>MGSHHHHHHTQPMPGKPAEDAENELDIRGLFRTLWAGKLWIIGMGLAFALIALAYTFFARQEWSSTAITDRPTVNMLGGYYSQQQFLRNLDVRSNMASADQPSVMDEAYKEFVMQLASWDTRREFWLQTDYYKQRMVGNSKADAALLDEMINNIQFIPGDFTRAVNDSVKLIAETAPDANNLLRQYVAFASQRAASHLNDELKGAWAARTIQMKAQVKRQEEVAKAIYDRRMNSIEQALKIAEQHNISRSATDVPAEELPDSEMFLLGRPMLQARLENLQAVGPAFDLDYDQNRAMLNTLNVGPTLDPRFQTYRYLRTPEEPVKRDSPRRAFLMIMWGIVGGLI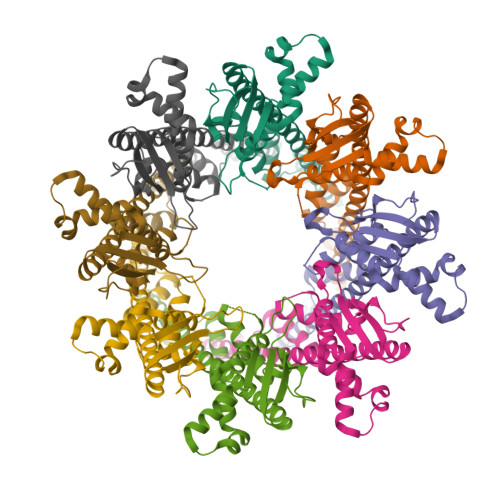GAGVALTRRCSK[32x]D-psicose | C6 H12 O6 | 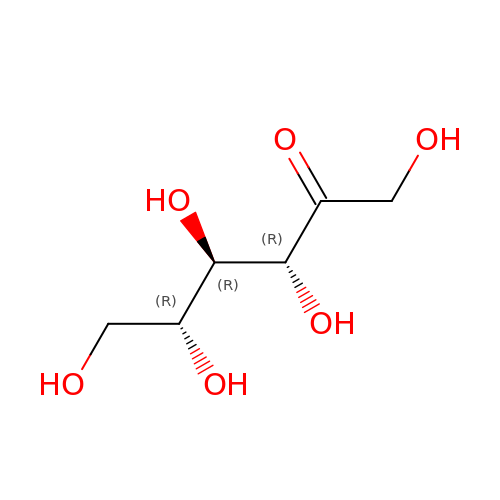BJHIKXHVCXFQLS-PUFIMZNGSA-N> KMNESDIWFEEKLQEVECEEQRLRKLHAVVETLVNHRKELALNTAQFAKSLAMLGSSEDNTALSRALSQLAEVEEKIEQLHQEQANNDFFLLAELLSDYI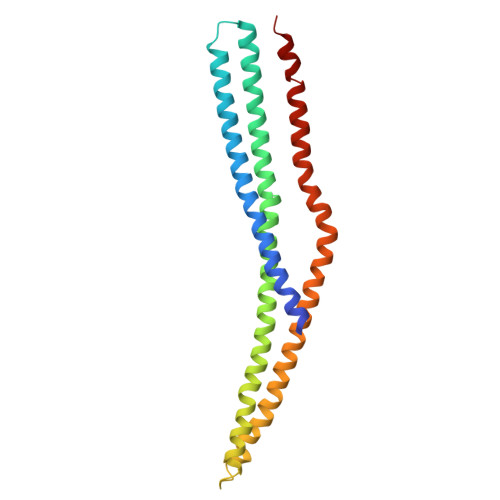RLLAIVRAAFDQRMKTWQRWQDAQATLQKKREAEARLLWANKPDKLQQAKDEILEWESRVTQYERDFERISTVVRKEVIRFEKEKSKDFKNHVIKYLETLLYSQQQLAKYWEAFLPEAKAIS>GMLKILATQFNGKLQTLTKQEDELFDVVRLLAQALVGQGKVYLDAYGEFEGLYPMLSDGPDQMKRVTKIKDHKTLHAVDRVLIFTPDTERSDLLASLARYDAWH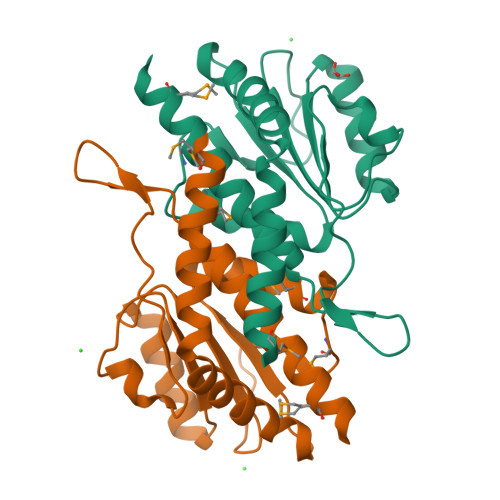TPYSIITLGDVTETLERSIAPLALKFDKGLLPAEDGSRHGLPSLALGAFLLTHILTQLQEMTEEWE[2x]> VTVDQDLLDAAGILPFEQVDIYDITNGARLTTYALPGERGSGVIGINGAAAHLVKPGDLVILVAYGVF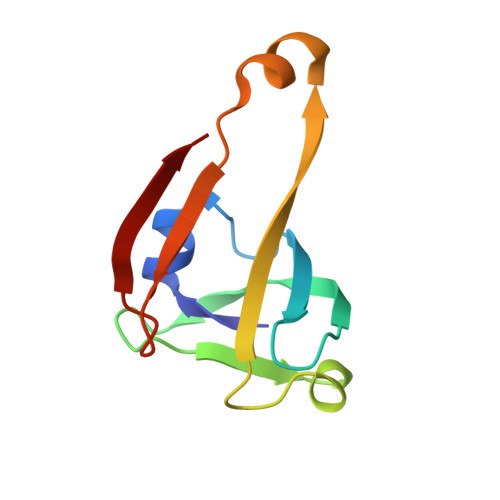DEEEARNLKPTVVLVDERNRILEVRKG>SNALQPNMRTRVCTVINNNIAHEWTLARIASELLMSPSLLKKKLREEETSYSQLLTECRMQRALQLIVIHGFSIKRVAVSCGY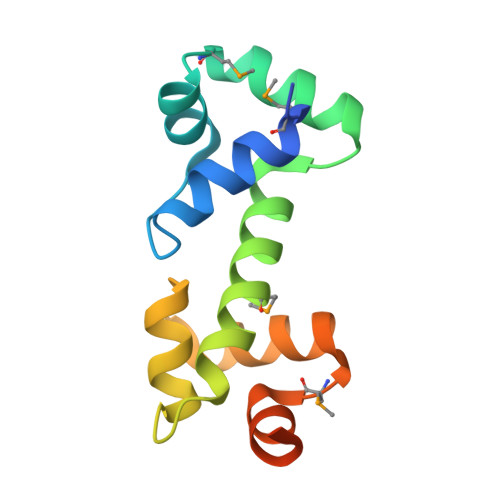HSVSYFIYVFRNYYGMTPTEYQERSAQRLSNRDSAAS[2x]> SNASVERVYQKKTQLEHILLRPDTYIGSVEPLTQFMWVYDEDVGMNCREVTFVPGLYKIFDEILVNAADNKQRDKNMTCIKVSIDPESNIISIWNNGKGIPVVEHKVEKVYVPALIFGQLLTSSNYDDDEKKVTGGRNGYGAKLCNIFSTKFTVETACKEYKHSFKQTWMNNMMKTSEAKIKHFDGEDYTCITFQPDLSKFKMEKLDKDIVALMTRRAYDLAGSCRGVKVMFNGKKLPVNGFRSYVDLYVKDKLDETGVALKVIHELANERWDVCLTLSEKGFQQISFVNSIATTKGGRHVDYVVDQVVGKLIEVVKKKNKAGVSVKPFQVKNHIWVFINCLIENPTFDSQTKENMTLQPKSFGSKCQLSEKFFKAASNCGIVESILNWVKFKAQTQ

Topoisomerase II (TOP2) enzymes are essential regulators of DNA topology during DNA transcription, replication, and repair. Topoisomerase IIβ (TOP2B) plays a role in transcriptional regulation and is expressed in all cell types including post-mitotic cardiomyocytes. Both isoforms catalyze the reaction, where one DNA duplex is passed through a transient double-strand DNA break in another DNA duplex. The ATPase domain of TOP2 is highly conserved between TOP2A and TOP2B and is composed of an N-terminal strap, a β-hairpin that is unique to eukaryotic TOP2, a GHKL ATPase domain that binds and hydrolyses ATP, and a transducer domain that conveys mechanical motion to the DNA binding and cleavage core of TOP2. Here we describe the development of the obex class of TOP2 inhibitors that bind to a previously unidentified druggable pocket in the TOP2 ATPase domain to act as allosteric catalytic inhibitors by locking the ATPase domain conformation with the capability of isoform-selective inhibition.

We have been unable to obtain crystal structures of nucleotide-free eukaryotic ATPase domains, and to our knowledge none have yet been described to date. Therefore, a comparison of the AMPPNP and AMPPNP + obex inhibitor structures reveal that the obex binding site is pre-formed in the ATP-bound state of TOP2, suggesting that topobexin (9) fits into TOP2B like a key into a lock and blocks subsequent conformational changes that could otherwise occur upon ATP hydrolysis. Residues surrounding the 5c pocket are largely unchanged from those observed in its absence, suggesting the ATP-bound state can easily accommodate 5c.> AMDIQPSVGFASRGSLLPGKVVEGLPVMALNVNNVDVNFFRVKPESLPAFISQWEYRNSLANWQSDKLLQMADLVYTGRFDLNPARNTREKLLLPLGDI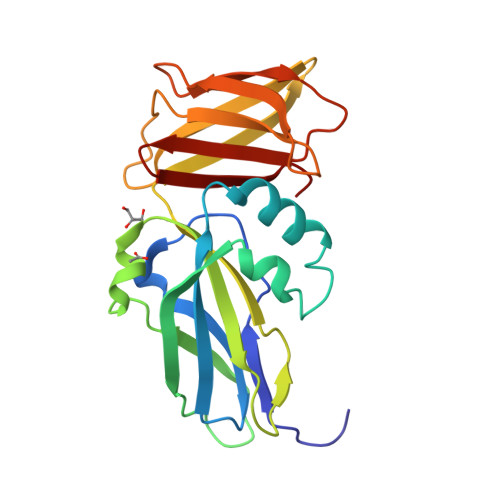KPLQQAGVYLAVMNQAGRYDYSNPATLFTLSDIGVSAHRYHNRLDIFTQSLENGAAQQGIEVSLLNEKGQTLTQATSDAQGHVQLENDKNAALLLARKDGQTTLLDLKL>[4x]MAKKTSSKGKLPPRVPNLIPYVGSFVSFAKNPVQFIIDNSKKYGDVFTATILGKEMTFLNHPKILDTFFKATDNELSLRDVYRFM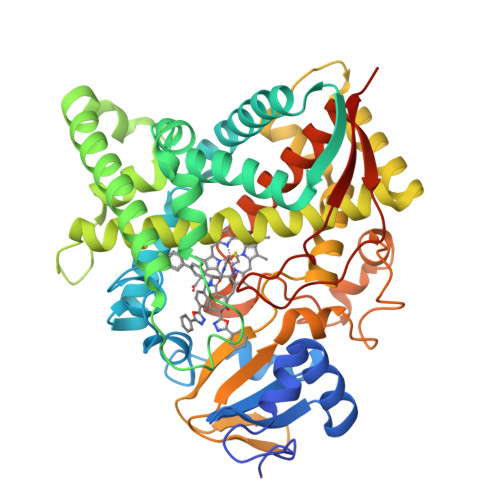RPVFGTGVVYDADSTERMMEQVKFVSSGLTTARFRVFVDIFEDEIAHKVKELGPEGTVDVAELMADLIIFTASRCLLGDEVRQYLSEKNLGKLYHDIDDGISPLSFFYPSLPAPKRDKARKAVGEIFQELLDKRREEHKKHPERLLDESKMDVVDHLLTQKYKDGQELTDVHRIGILIAGLFAGQHTSSITSSWTLMNVISNKKVLEKVRKEQEEIMGSDKVLDYDKVMKMDYLEACMKEALRMYPPLIMIMRMARKPRECEQYIIPKGNILVVSPSVAGRCTDTYTNPDVFDPERLTERKEHEKFKYGAVPFGAGRHKCIGENFALLQVKSIISILLRYFDMEYIGKIPDPSYTSLVVGPSPPTRMRYKLRKQQHHHHHH>[2x]MHHHHHHAAGIPMNNPAIKRIGNHITKSPEDKREYRGLELANGIKVLLISDPTTDKSSAALDVHIGSLSDPPNIAGLSHFLQHMLFLGTKKYPKENEYSQFLSEHAGSSNAFTSGEHTNYYFDVSHEHLEGALDRFAQFFLSPLFDESAKDREVNAVDSEHEKNVMNDAWRLFQLEKATGNPKHPFSKFGTGNKYTLETRPNQEGIDVRQELLKFHSAYYSSNLMAVVVLGRESLDDLTNLVVKLFSEVENKNVPLPEFPEHPFQEEHLKQLYKIVPIKDIRNLYVTFPIPDLQKYYKS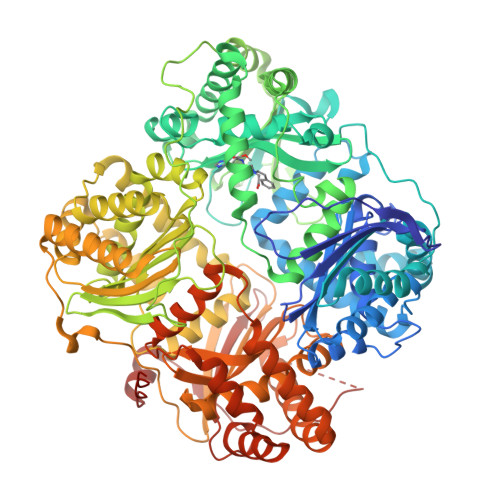NPGHYLGHLIGHEGPGSLLSELKSKGWVNTLVGGQKEGARGFMFFIINVDLTEEGLLHVEDIILHMFQYIQKLRAEGPQEWVFQELKDLNAVAFRFKDKERPRGYTSKIAGILHYYPLEEVLTAEYLLEEFRPDLIEMVLDKLRPENVRVAIVSKSFEGKTDRTEEWYGTQYKQEAIPDEVIKKWQNADLNGKFKLPTKNEFIPTNFEILPLEKEATPYPALIKDTAMSKLWFKQDDKFFLPKANLNFEFFSPFAYVDPLHSNMAYLYLELLKDSLNEYAYAAELAGLSYDLQNTIYGMYLSVKGYNDKQPILLKKIIEKMATFEIDEKRFEIIKEAYMRSLNNFRAEQPHQHAMYYLRLLMTEVAWTKDELKEALDDVTLPRLKAFIPQLLSRLHIEALLHGNITKQAALGIMQMVEDTLIEHAHTKPLLPSQLVRYREVQLPDRGWFVYQQRNEVHNNSGIEIYYQTDMQSTSENMFLELFAQIISEPAFNTLRTKEQLGYIVFSGPRRANGIQGLRFIIQSEKPPHYLESRVEAFLITMEKSIEDMTEEAFQKHIQALAIRRLDKPKKLSAESAKYWGEIISQQYNFDRDNTEVAYLKTLTKEDIIKFYKEMLAVDAPRRHKVSVHVLAREMDSNPVVGEFPAQNDINLSQAPALPQPEVIQNMTEFKRGLPLFPLVKPHINFMAAKL>[4x]VSDLPPSVDWRQKGAVTGVKDQGKCGSCWAFSTVVSVEGINAIRTGSLVSLSEQELIDCDTADNDGCQGGLMDNAFEYIKNNGGLITEAAYPYRAARGTCNVARAAQNSPVVVHIDGHQDVPANSEEDLARAVANQPVSVAVEASGKAFMFYSEGVFTGECGTELDHGVAVVGYGVAEDGKAYWTVKNSWGPSWGEQGYIRVEKDSGASGGLCGIAME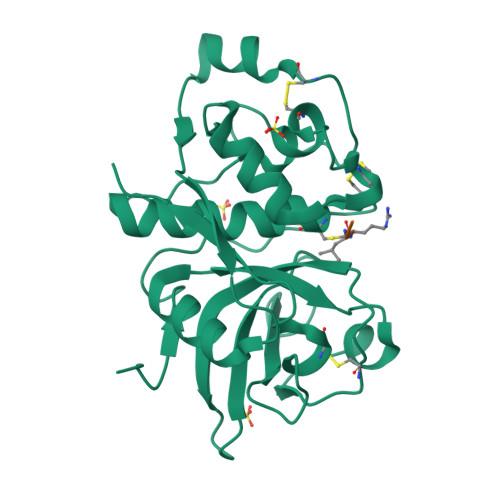ASYPVKTYSKPKPTPRRALGARESLNSSSVDKLAAALEHHHHHH> MFSAKKRDKCIGEMSEKQLDLLVIGGGITGAGIALDAQVRGIQTGLVEMNDFASGTSSRSTKLVHGGLRYLKQFEIKLVAEVGKERAIVYENAPHVTTPEWMLLPIFKDGTFGKFSTSLGLKVYDYLADVRKDERRYMLNEKQTLEKEPLLRKENLKGGGIYVEYRTDDARLTLEIMKEAVARGAVALNYMKVESFIYDQGKVVGVVAKDRLTDTTHTIYAKKVVNAAGPWVDTLREKDRSKHGKYLKLSKGV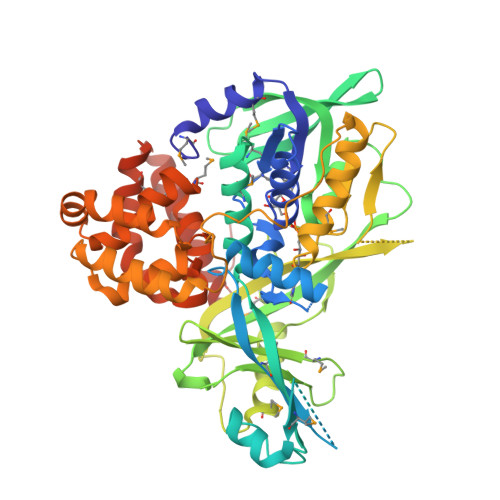HLVVDQSRFPLRQAVYFDTESDGRMIFAIPREGKTYIGTTDTFYDKDIASPRMTVEDRDYILAAANYMFPSLRLTADDVESSWAGLRPLIHEEGKKASEISRKDEIFFSDSGLISIAGGKLTGYRKMAERTVDAVAQGLNVNEPCTTAAIRLSGGLAEGAQGFPRFLDEASRKGAKLGFDADEVRRLAKLYGSNVDHVLNYAYEGKEEAEHYGLPALLLGQLQYGVEQEMVATPLDFFVRRTGALFFNISLVHQWKEAVLRWMAEEFSWTEEEKTRFQNELETELKMAVDPLFQVEPTTVLEHHHHHH> TEFKAGSAKKGATLFKTRCLQCHTVE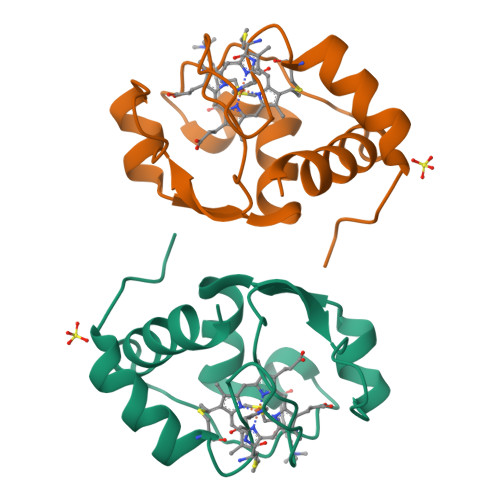KGGPHKVGPNLHGIFGAHSGQAEGYSYTDAIIKKNVLWDENNMSEYLTNPKKYIPGTKMASGGLKKEKDRNDLITYLKKAAE Protoglobin (Pgb) is a recently discovered haem-protein with distinct structural and functional features that make it unique within the globin superfamily. The MaPgb* structure can be considered as an expanded version of the 3/3 helical sandwich typical of “classical” globins (i.e. Mb), with an additional N-terminal extension, built by a 20-residue loop, followed by the Z-helix, which precedes the globin-fold conserved A-helix. Residues belonging to the Z-helix contribute to formation of the Pgb homodimer, which is centered on the intermolecular four-helix bundle built by the G- and H-helices of the two subunits. Thus, in Pgb the access of diatomic ligands, such as O2, CO, and NO, to the haem is granted by two orthogonal apolar tunnels that reach the haem distal region from entry sites at the B/G and B/E helix interfaces.

The Phe(93)E11Leu mutation does not prevent the insertion of the Trp(60)B9 side chain into the distal site and the stabilization of the haem-Fe(III)-bound cyanide. Thus, the ligand sensing capability of the E11 residue, reflected by Trp(60)B9 conformational changes, does not require specifically a Phe residue. In the Phe(93)E11Leu mutant structure (three MaPgb* chains in the asymmetric unit), however, the haem-Fe(III)-bound cyanide molecule is stabilized only by the H-bond provided by the Nε2 atom of Trp(60)B9 (∼2.8 Å). Indeed, the orientation of the Tyr(61)B10 side chain matches that found in the MaPgb(III)-cyanide structure, but its side chain is slightly shifted away from the center of the haem distal cavity, its OH group being at ∼4 Å from the cyanide N atom. Analysis of the crystal structure shows that the mutated Leu(93)E11 side chain imposes to the Tyr(61)B10 side chain a slightly unfavorable location for H-bonding to the haem-bound cyanide (the OH group of residue Tyr(61)B10 falls at 4.25 Å on average from the haem-bound cyanide, in the three independent subunits). However, no intervening steric impediments are present for the formation of such H-bond. Indeed, inspection of difference Fourier maps reveals the presence of a positive electron density peak (∼3.8 σ) between the Tyr(61)B10 side chain and the haem-bound cyanide in one of three Phe(93)E11Leu mutant molecules present in the crystal asymmetric unit. Such observation suggests that even in the static crystal environment a fraction of the mutant molecules may stabilize the haem-bound cyanide through two H-bonds. The only exception is the Phe(93)E11Leu mutant, where two H-bonding interactions are expected from the dissociation kinetics measurements, while only one, to the Nε2 atom of Trp(60)B9, is found in the crystal structure of the cyanide derivative.

>[3x]MSVEKIPGYTYGETENRAPFNLEDLKLLKEAVMFTAEDEEYIQKAGEVLEDQVEEILDTWYGFVGSHPHLLYYFTSPDGTPNEKYLAAVRKRLSRWILDTSNRSYDQAWLDYQYEIGLRHHRTKKNQTDNVESVPNIGYRYLVAFIYPITATMKPFLARKGHTPEEVEKMYQAWFKATTLQVALWSYPYVKYGDF1-[2-[4-(4-oxidanylidene-3,7-dihydropyrrolo[2,3-d]pyrimidin-5-yl)-1,2,3-triazol-1-yl]ethyl]guanidine 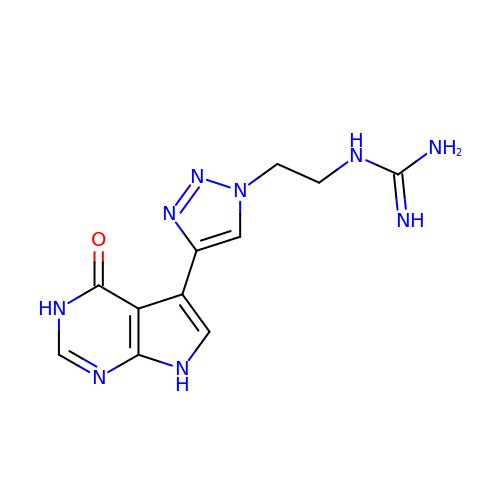| C11 H13 N9 O | XNDGGOMEAZTNJB-UHFFFAOYSA-N> GGGFCTSAGALWIYPTNCPVRDYQLHISRAALFCNTLVCLPTGLGKTFIAAVVMYNFYRWFPSGKVVFMAPTKPLVTQQIEACYQVMGIPQSHMAEMTGSTQASTRKEIWCSKRVLFLTPQVMVNDLSRGACPAAEIKCLVIDEAHKALGNYAYCQVVRELVKYTNHFRILALSATPGSDIKAVQQVITNLLIGQIELRSEDSPDILTYSHERKVEKLIVPLGEELAAIQKTYIQILESFARSLIQRNVLMRRDIPNLTKYQIILARDQFRKNPSPNIVGIQQGIIEGEFAICISLYHGYELLQQMGMRSLYFFLCGIMDGTKGMTRSKNELGRNEDFMKLYNHLECMFARTRSTSANGISAIQQGDKNKKFVYSHPKLKKLEEVVIEHFKSWNAENTTEKKRDETRVMIFSSFRDSVQEIAEMLSQHQPIIRVMTFVGHASGKSTKGFTQKEQLEVVKQFRDGGYNTLVSTCVGEEGLDIGEVDLIICFDSQKSPIRLVQRMGRTGRKRQGRIVIILSEGREERIYNQSQSNKRSIYKAISSNRQVLHFYQRSPRMVPDGINPKLHKMFITH

FANCM is crucial in genome maintenance, functioning in the Fanconi anemia (FA) pathway, alternative lengthening of telomeres (ALT), and replication fork protection. FANCM recognizes branched DNA structures and promotes their remodeling through ATP-dependent branch migration. Here we present crystal structures of FANCM’s N-terminal ATP-dependent translocase domain (2.2 Å) and C-terminal FAAP24-bound region (2.4 Å), both complexed with branched DNA. The N-terminal translocase domain specifically recognizes DNA junctions through multiple key elements, while the C-terminal FAAP24-binding domain engages adjacent double-stranded DNA.

To understand how FANCM identifies DNA damage sites, we determined the crystal structure of its N-terminal translocase domain bound to branched DNA at 2.2 Å resolution. This high-resolution view reveals a sophisticated molecular machine built around three core elements: two RecA-like domains (RecA1 and RecA2) that form the motor unit, connected by a specialized insert domain (Hel2i) that recognizes DNA branch points. In particular, we observed that the opening angle between RecA2 and Hel2i is markedly reduced in FANCM compared to the other enzymes, all of which process double-stranded nucleic acids. This tighter configuration is likely key to the binding of the branchpoint by FANCM, as compared to a looser configuration, which permits the passage of double-stranded molecules over the RecA1-RecA2 interface in structurally related proteins. While the N-terminal α-helix maintains a comparable trajectory in FANCM, the C-terminal helix adopts a distinct orientation, positioned at ~130° relative to the first helix and traversing an alternative molecular surface. Because of this modified and distinct pincer architecture, we renamed this sequence as the “mincer” domain. Our crystal structures revealed how FANCM achieves this efficiency through precise DNA contacts. First, the N-terminal domain creates a positively charged channel that grips DNA at the branchpoint (Figs. 5F and EV4). Two key residues in the Hel2i domain—H369 and Y332—make specific contacts with the 5′ and 3′ sides of the junction respectively (inset 1). The newly identified mincer domain provides additional structure-specific recognition through a long helix that contacts the 3′ DNA arm (inset 2).> MTRDLAPALQALSPLLGSWAGRGAGKYP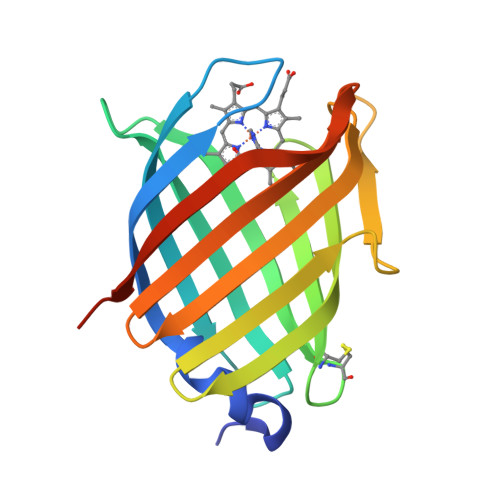TIRPFEYLEEVVFAHVGKPFLTYTQQTRAVADGKPLHSETGYLRVCRPGCVELVLAHPSGITEIEVGTYSVTGDVIELELSTRADGSIGLAPTAKEVTALDRSYRIDGDELSYSLQMRAVGQPLQDHLAAVLHRQRRSHHHHHH> MNIFRLTGDLSHLAAIIILLLKIWKSRSCAGISGKSQLLFALVFTTRYLDLFTSFISLYNTSMKLIYIACSYATVYLIYMKFKATYDGNHDTFRVEFLIVPVGGLSFLVNHDFSPLEILWTFSIYLESVAILPQLFMISK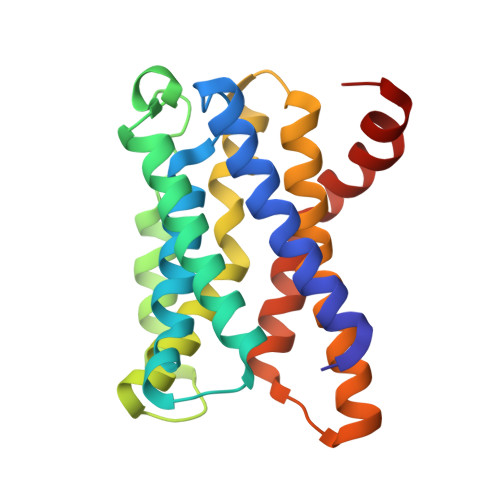TGEAETITTHYLFFLGLYRALYLVNWIWRYYFEGFFDLIAVVAGVVQTVLYCDFFYLYVTKVLKGKK> EVKQENRLLNESESSSQGLLGYYFSDLNFQAPMVVTSSTTGDLSIPSSELENIPSENQYFQSAIWSGFIKVKKSDEYTFATSADNHVTMWVDDQEVINKASNSNKIRLEKGRLYQIKIQYQRENPTEKGLDFKLYWTDSQNKKEVISSDNLQLPELKQKSSNSRKKRSTSAGPTVPDRDNDGIPDSLEVEGYTVDVKNKRTFLSPWISNIHEKKGLTKYKSSPEKWSTASDPYSDFEKVTGRIDKNVSPEARHPLVAAYPIVHVDMENIILSKNEDQSTQNTDSQTRTISKNTSTSRTHTSEVHGNAEVHASFFDIGGSVSAGFSNSNSSTVAIDHSLSLAGERTFAETMGLNTADTARLNANI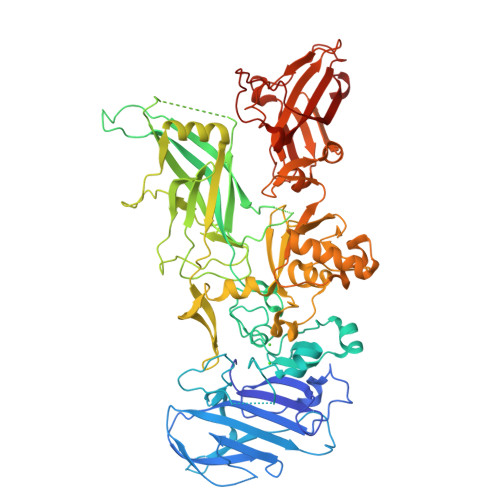RYVNTGTAPIYNVLPTTSLVLGKNQTLATIKAKENQLSQILAPNNYYPSKNLAPIALNAQDDFSSTPITMNYNQFLELEKTKQLRLDTDQVYGNIATYNFENGRVRVDTGSNWSEVLPQIQETTARIIFNGKDLNLVERRIAAVNPSDPLETTKPDMTLKEALKIAFGFNEPNGNLQYQGKDITEFDFNFDQQTSQNIKNQLAELNATNIYTVLDKIKLNAKMNILIRDKRFHYDRNNIAVGADESVVKEAHREVINSSTEGLLLNIDKDIRKILSGYIVEIEDTEGLKEVINDRYDMLNISSLRQDGKTFIDFKKYNDKLPLYISNPNYKVNVYAVTKENTIINPSENGDTSTNGIKKILIFSKKGYEIG> MTQFKEIEKTTDFKNHSLP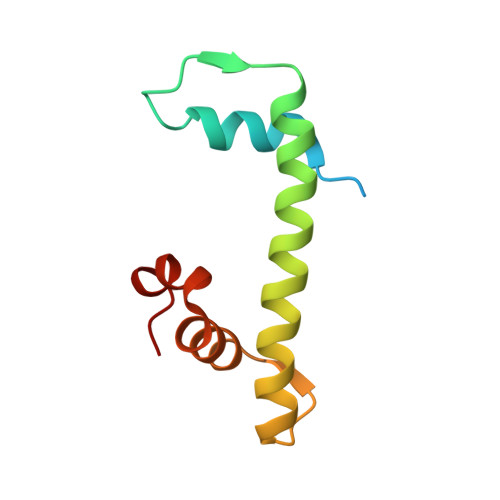LARIKKIMKADEDVRMISAEAPVVFARACEMFILELTLRSWNHTEENKRRTLQKNDIAAAVTRTDIFDFLVDIVPR{3-[3-(3,4-DIMETHOXY-PHENYL)-1-(1-{1-[2-(3,4,5-TRIMETHOXY-PHENYL)-BUTYRYL]-PIPERIDIN-2YL}-VINYLOXY)-PROPYL]-PHENOXY}-ACETIC ACID 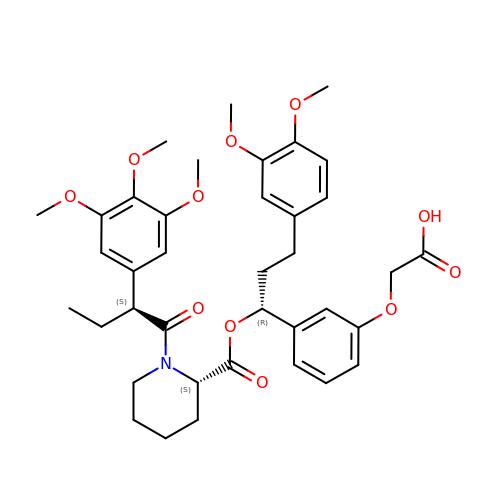| C38 H47 N O11 | XCCRAOPQCACRFC-OIFRRMEBSA-N> MKRRWKKNFIAVSAANRFKKISSSGALENLYFQGEAPVMEGSTGFDGDATTFFA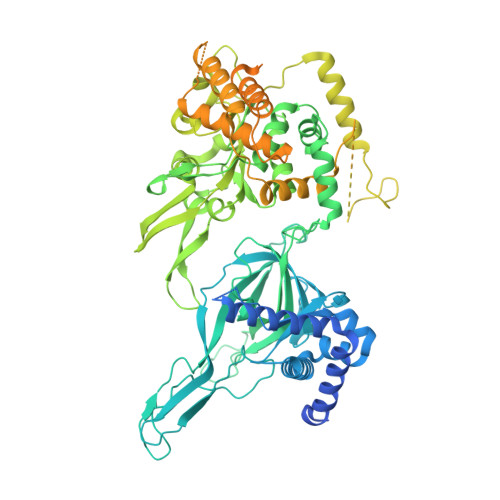PDAVFGDRVRRFQEFLDTFTSYRDSVRSIQVYNSNNAANYNDDQDDADERDLLGDDDGDDLEKEKKAASSTSLNILPHRIIISLDDLREFDRSFWSGILVEPAYFIPPAEKALTDLADSMDDVPHPNASAVSSRHPWKLSFKGSFGAHALSPRTLTAQHLNKLVSVEGIVTKTSLVRPKLIRSVHYAAKTGRFHYRDYTDATTTLTTRIPTPAIYPTEDTEGNKLTTEYGYSTFIDHQRITVQEMPEMAPAGQLPRSIDVILDDDLVDKTKPGDRVNVVGVFKSLGAGGMNQSNSNTLIGFKTLILGNTVYPLHARSTGVAARQMLTDFDIRNINKLSKKKDIFDILSQSLAPSIYGHDHIKKAILLMLMGGVEKNLENGSHLRGDINILMVGDPSTAKSQLLRFVLNTASLAIATTGRGSSGVGLTAAVTTDRETGERRLEAGAMVLADRGVVCIDEFDKMTDVDRVAIHEVMEQQTVTIAKAGIHTTLNARCSVIAAANPVFGQYDVNRDPHQNIALPDSLLSRFDLLFVVTDDINEIRDRSISEHVLRTHRYLPPGYLEGEPVRERLNLSLAVGEDADINPEEHSNSGAGVENEGEDDEDHVFEKFNPLLQAGAKLAKNKGNYNGTEIPKLVTIPFLRKYVQYAKERVIPQLTQEAINVIVKNYTDLRNDDNTKKSPITARTLETLIRLATAHAKVRLSKTVNKVDAKVAANLLRFALLGEDIGNDIDEEESEYEEALSKRSPQKSPKKRQRVRQPASNSGSPIKSTPRRSTASSVNATPSSARRILRFQDDEQNAGEDDNDIMSPLPADEEAELQRRLQLGLRVSPRRREHLHAPEEGSSGPLTEVGTPRLPNVSSAGQDDEQQQSVISFDNVEPGTISTGRLSLISGIIARLMQTEIFEEESYPVASLFERINEELPEEEKFSAQEYLAGLKIMSDRNNLMVADDKVWRV>[3x]RGSHHHH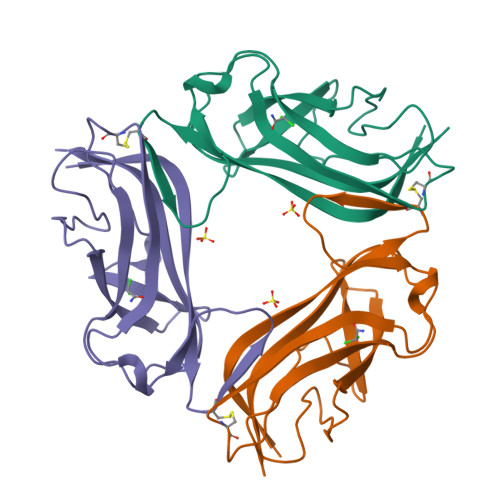HHGSFTPSGTTGTTKLTVTEKCQVRVGDLTVAKTRGQLTDAAPIGPVTVQALGCDARQVALKADTDNFEQGKFFLISDNNRDKLYVNIRPTDNSAWTTDNGVFYKNDVGSWGGIIGIYVDGQQTNTPPGNYTLTLTGGYWAK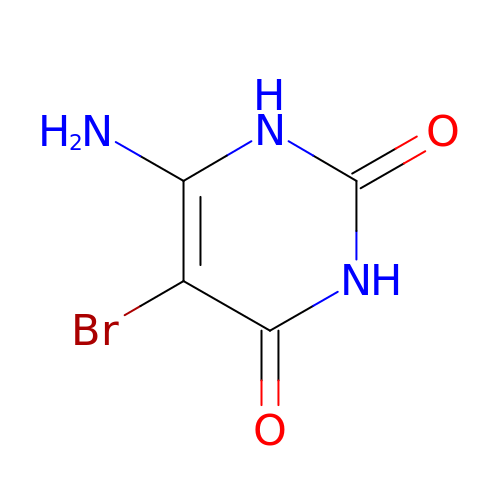6-amino-5-bromo-1,2,3,4-tetrahydropyrimidine-2,4-dione | C4 H4 Br N3 O2 | FSLBEEVCUZFKRL-UHFFFAOYSA-N> AQTVPYGIPLIKADKVQAQGFKGANVKVAVLDTGIQASHPDLNVVGGASFVAGEAYNTDGNGHGTHVAGTVAALDNTTGVLGVAPSVSLYAVKVLNSSGSGSYSGIV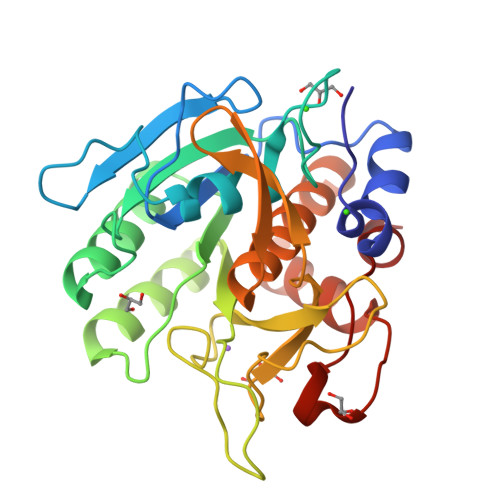SGIEWATTNGMDVINMSLGGASGSTAMKQAVDNAYARGVVVVAAAGNSGSSGSTNTIGYPAKYDSVIAVGAVDSNSNRASFSSVGAELEVMAPGAGVYSTYPTNTYATLNGTSMASPHVAGAAALILSKHPNLSASQVRNRLSSTATYLGSSFYYGKGLINVEAAAQ>[2x]MVRILLINSDKPEPIQFFQKDKETNDSINISVITRSCYAPLYSHWADHVYIVDDVTDLTVMKSLMLEILKVGPIDHIVSTTEKSILTGGFLRSYFGIAGPGFETALYMTNKLAMKTKLKMEGIPVADFLCVSQVEDIPAAGEKLGWPIIVKPALGSGALNTFIIHSLDHYEDLYSTSGGLGELKKNNSLMIAEKCIEMEEFHCDTLYADGEILFVSI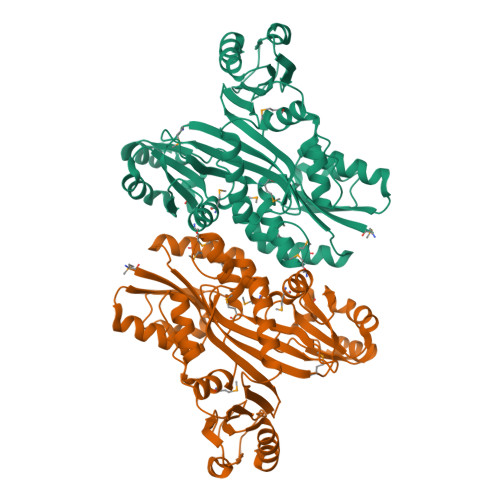SKYTVPLLKGMAKIQGSFILSQNDPVYAEILELQKSVAQAFRITDGPGHLEIYRTHSGELIVGEIAMRIGGGGISRMIEKKFNISLWESSLNISVYRDPNLTVNPIEGTVGYFSLPCRNGTIKEFTPIEEWEKLAGILEVELLYQEGDVVDEKQSSSFDLARLYFCLENENEVQHLLALVKQTYYLHLTEDHMMNQ>[2x]GT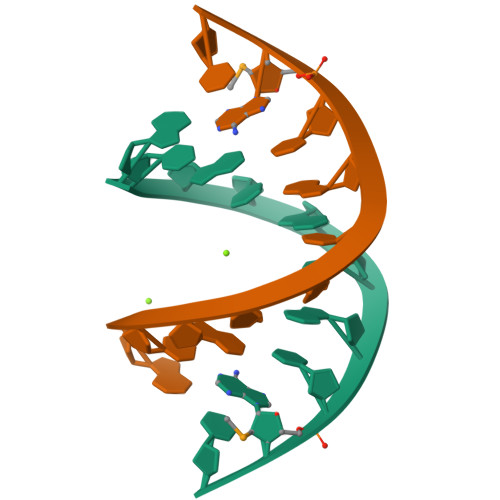ACGCGTAC(R)-pyridin-4-yl[4-(2-pyrrolidin-1-ylethoxy)phenyl]methanol | 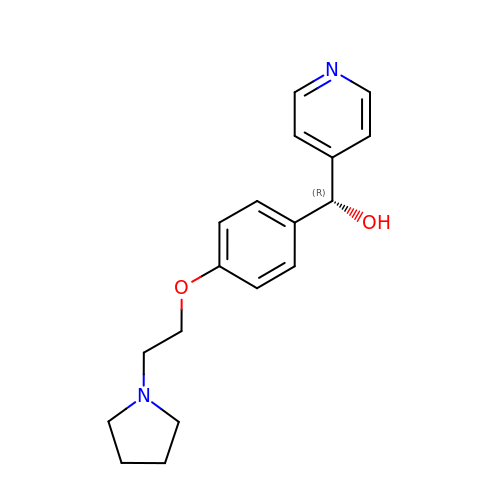C18 H22 N2 O2 | QQRJWLDQBNAQCC-GOSISDBHSA-N> MAKAHIELTINGHPVEALVEPRTLLIHFIRE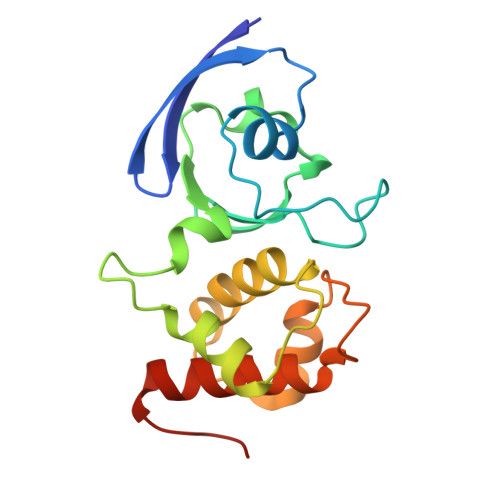QQNLTGAHIGCDTSHCGACTVDLDGMSVKSCTMFAVQANGASITTIEGMAAPDGTLSALQEGFRMMHGLQCGYCTPGMIMRSHRLLQENPSPTEAEIRFGIGGNLCRCTGYQNIVKAIQYAAAKINGVPFEEAAE2,4-dibromo-6-{[(2-nitrobenzene-1-carbonyl)amino]methyl}phenyl 2-cyanobenzoate 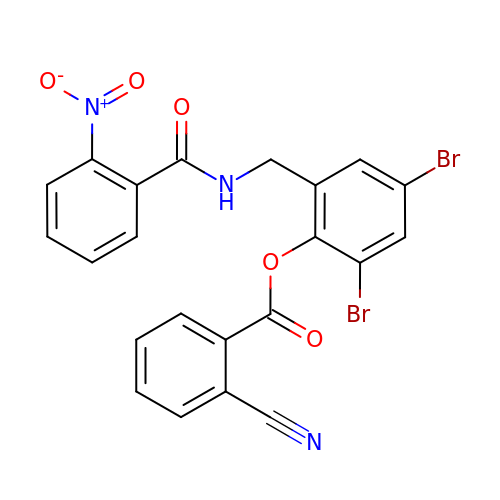| C22 H13 Br2 N3 O5 | PYKOCDMESJAHAB-UHFFFAOYSA-N> GEEWGP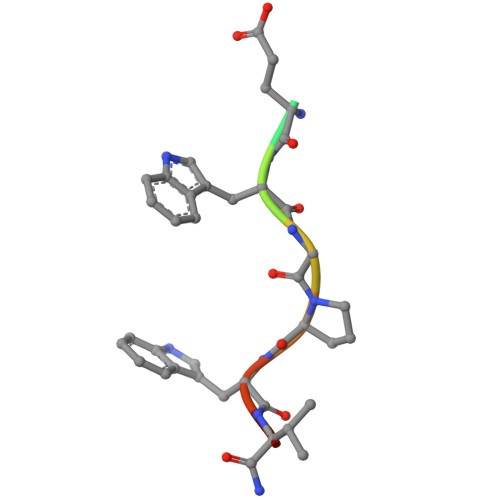WVX> MAHHHHHHMPSLKSSKRYNKYTILQVVPALVSGGVERGTIEVAKYLKILGHTPIIISVGGTLVKELDKEDILHIEMNSNSKNPFVILNNAKLIAEIIKKYNVDIVHTRSRAPAWSSYLATKWTNAKFLTTFHGVYNIPNSFKKYYNSIMLKGKKVVAV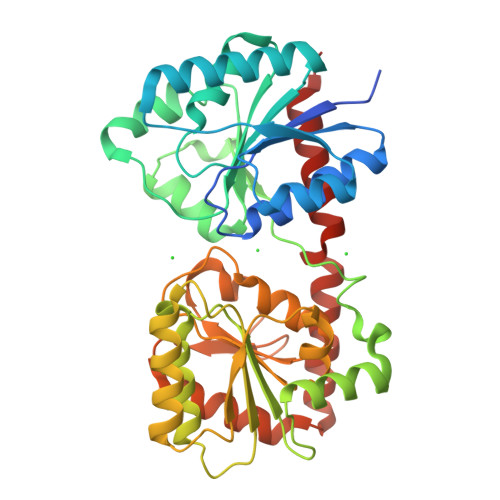SNFVKQHLLENYKIDEDKIVVIERGVNCDYFDPANLTPEKLEKCCEKYDVPSNVPIILMPSRMTSWKGHLVLVEALSKLKHRDFYCLMVGDISRHPNFTNRVKELIANLKLQNKIQIFGNDSDIINLYGISDIIISASIEPEAFGRTIIEGQAMKKLVIATNIGGAVETINNNITGFHVEPNNAEALAQKIDYCFSILGTDLAKKIQEAARHTVINNFSLNLMLRKNLEIYKEILKNSHN>[2x]SPYSSDTTPCCFAYIARPLPRAHIKEYFYTSGK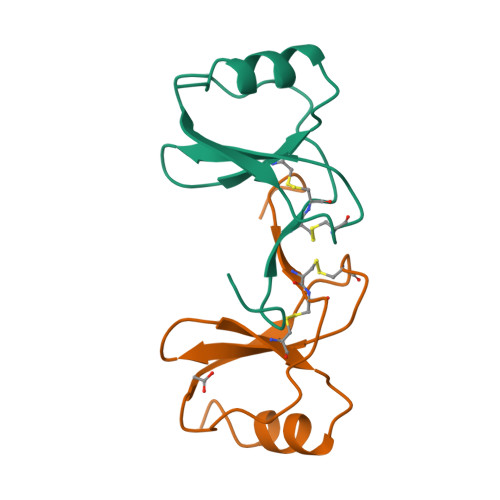CSNPAVVFVTRENRQVCANPEKKWVREYINSLEMS> NSNNKRAPYWTNTEKMEKRLHAVPAANTVKFRCPAGGNPMPTMRWLKNGKEFKQEHRIGGYKVRNQHWSLIMESVVPSDKGNYTCVVENEYGSINHTYHLDVVERSRHRPILQAGLPANASTVVGGDVEFVCKVYSDAQPHIQWIKHVEKNGSKYGPDGLPYLKVLKAAGVNTTDKEIEVLYIRNVTFEDAGEYTCLAGNSIGISFHSAWLTVLPAP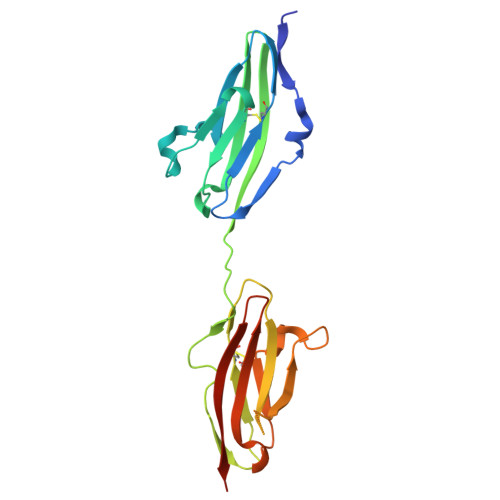GRE>[2x]MRADVKPVTVKLVDSQATMETRSLFAFMQEQRRHSIMFGHQHETTQGLTITRTDGTQSDTFNAVGDFAAVYGWDTLSIVAPKAEGDIVAQVKKAYARGGIITVSSHFDNPKTDTQKGVWPVGTSWDQTPAVVDSLPGGAYNPVLNGYLDQVAEWANNLKDEQGRLIPVIFRLYHENTG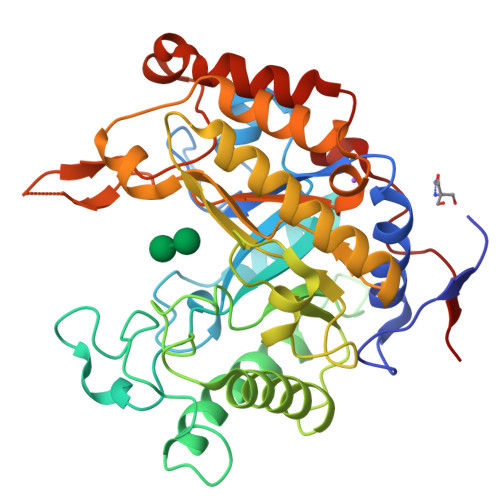SWFWWGDKQSTPEQYKQLFRYSVEYLRDVKGVRNFLYAYSPNNFWDVTEANYLERYPGDEWVDVLGFDTYGPVADNADWFRNVVANAALVARMAEARGKIPVISGIGIRAPDIEAGLYDNQWYRKLISGLKADPDAREIAFLLVWRNAPQGVPGPNGTQVPHYWVPANRPENINNGTLEDFQAFYADEFTAFNRDIEQVYQRPTLIVK ThiC, the enzyme discussed here, catalyses the complex rearrangement of aminoimidazole ribonucleotide (AIR) to 4-amino-5-hydroxymethyl-2-methylpyrimidine phosphate (HMP-P) in the thiamin biosynthetic pathways of bacteria and plants 17 and is an example of a non-canonical radical SAM enzyme. The CX2CX4C motif of ThiC varies from the canonical radical SAM motif and is located near the C terminus of the sequence. The homodimeric structure of Caulobacter crescentus ThiC (CcThiC) showed a (β/α)8-barrel fold and suggested that the cluster-binding domain, which was disordered, resides near the C terminus and inserts into the active site of an adjacent protomer through domain swapping. The cluster-binding domain inserts into the active site of an adjacent catalytic domain through domain swapping as previously predicted.

One structure of CcThiC and one structure of AtThiC stand apart and provide insight into conformational changes occurring in ThiC. In the holo CcThiC structure, the entire C-terminal cluster-binding domain and [4Fe-4S] cluster are clearly defined; however, the cluster-binding domain extends away from the active site and the cluster itself is ~25 Å from its active site location. (v) The positioning of the [4Fe-4S] cluster in the active site, along with two structures lacking SAH or L-Met and 5′-dAdo, suggests that the tethered ThiC cluster-binding domain moves into the ThiC active site to initiate catalysis and out of the active site to release products.

> GHMNIQSTIKAVAETISTGPIPGSRKVYQAGELFPELRVPFREVAVHPSANEPPVTIYDPSGPYSDPAIQIDIEKGLPRTREALVVARGDVEEVADPRQVKPEDNGFAQGKHLAPEFPDTGRKIYRAKPGKLVTQLEYARAGIITAEMEYVAIRENLRREQDRPCVRDGEDFGASIPDFVTPEFVRQEIARGRAIIPANINHGELEPMAIGRNFLVKINANIGNSAVLSTVADEVDKLVWATRWGADTVMDLSTGRNIHNIRDWIIRNSSVPIGTVPIYQALEKVNGVAEDLNWEVFRDTLIEQCEQGVDYFTIHAGVRLPFIPMTAKRVTGIVSRGGSIMAKWCLAHHKENFLYERFDEICEIMRAYDVSFSLGDGLRPGSTADANDEAQFSELRTLGELTKVAWKHGVQVMIEGPGHVAMHKIKANMDEQLKHCHEAPFYTLGPLTTDIAPGYDHITSAIGAAMIGWFGTAMLCYVTPKEHLGLPDRDDVKTGVITYKLAAHAADLAKGHPGAAMWDDAISRARFEFRWEDQFNLGLDPETARKFHDETLPKEAHKTAHFCSMCGPKFCSMKISQEVRDFAAGKAPNSAELGMAEMSEKFREQGSEIYLKTE> VVGGEDAKPGQFPWQVVLNGKVDAFCGGSIVNEKWIVTAAHCVETGVKITVVAGEHNIEETEHTEQKRNVIRIIPHHNYNAAINTYNHDIALLELDEPLVLNSYVTPICIADKEYTNIFLKFGSGYVSGWGRVFHKGRSALVLQYLRVPLVDRATCLRSTKFTIYNNMFCAGFHEGGRDSCQGDSGGPHVTEVEGTSFLTGIISWGEECAMKGKYGIYTK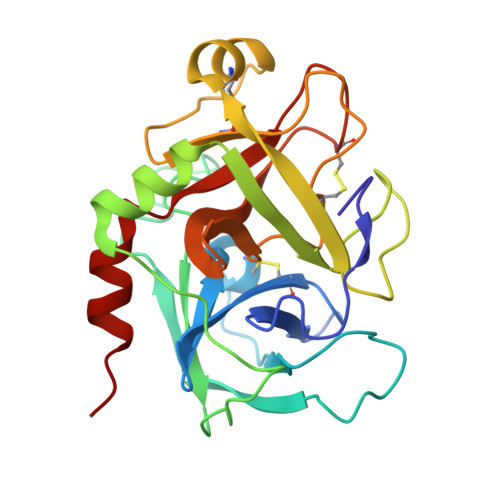VSRYVNWIKEKTKLT> MGNFANRKPHVVMIPYPVQGHINPLFKLAKLLHLRGFHITFVNTEYNHKRLLKSRGPKAFDGFTDFNFESIPDGLTPMEGDGDVSQDVPTLCQSVRKNFLKPYCELLTRLNHSTNVPPVTCLVSDCCMSFTIQAAEEFELPNVLYFSSSACSLLNVMHFRSFVERGIIPFKDESYLTNGCLETKVDWIPGLKNFRLKDIVDFIRTTNPNDIMLEFFIEVADRVNKDTTILLNTFNELESDVINALSSTIPSIYPIGPLPSLLKQTPQIHQLDSLDSNLWKEDTECLDWLESKEPGSVVYVNFGSTTVMTPEQLLEFAWGLANCKKSFLWIIRPDLVIGGSVIFSSEFTNEIADRGLIASWCPQDKVLNHPSIGGFLTHCGWNSTTESICAGVPMLCWPFFADQPTDCRFICNEWEIGME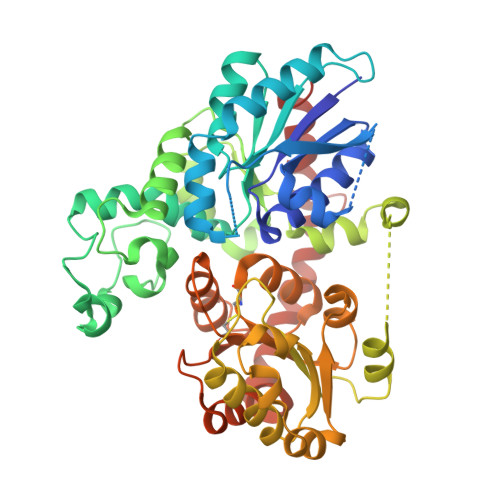IDTNVKREELAKLINEVIAGDKGKKMKQKAMELKKKAEENTRPGGCSYMNLNKVIKDVLLKQN> LDKVYQMKSKPRGYCLIINNH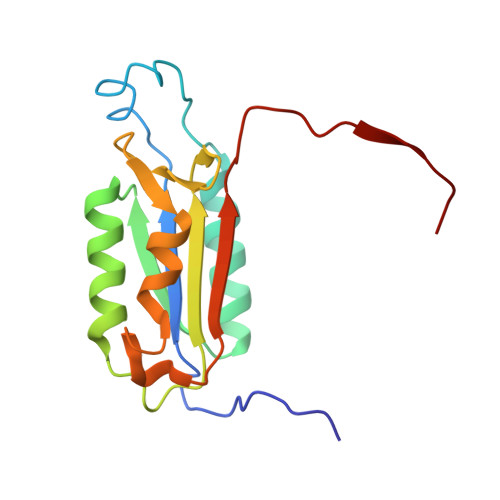NFAKAREKVPKLHSIRDRNGTHLDAGALTTTFEELHFEIKPHHDCTVEQIYEILKIYQLMDHSNMDCFICCILSHGDKGIIYGTDGQEAPIYELTSQFTGLKCPSLAGKPKVFFIQACQGDNYQKGIPVETD>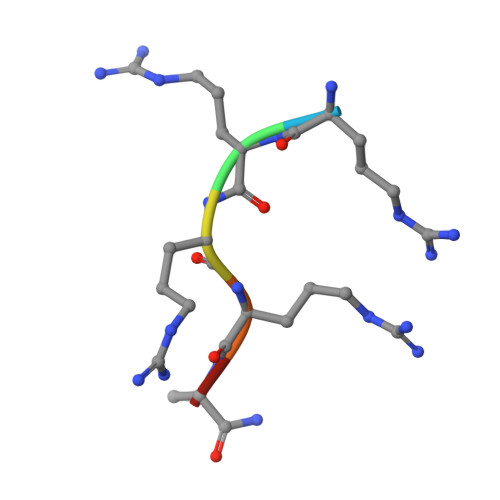 RRRRAX> SQTVHFQGNPVTVANSIPQAGSKAQTFTLVAKDLSDVTLG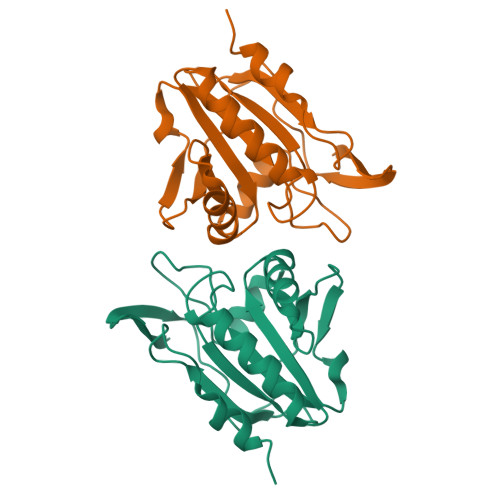QFAGKRKVLNIFPSIDTGVSAASVRKFNQLATEIDNTVVLCISADLPFAQSRFCGAEGLNNVITLSTFRNAEFLQAYGVAIADGPLKGLAARAVVVIDENDNVIFSQLVDEITTEPDYEAALAVLKA N-[(1S,2R)-1-benzyl-3-{[(1S)-2-(cyclohexylamino)-1-methyl-2-oxoethyl]amino}-2-hydroxypropyl]-3-(pentylsulfonyl)benzamide 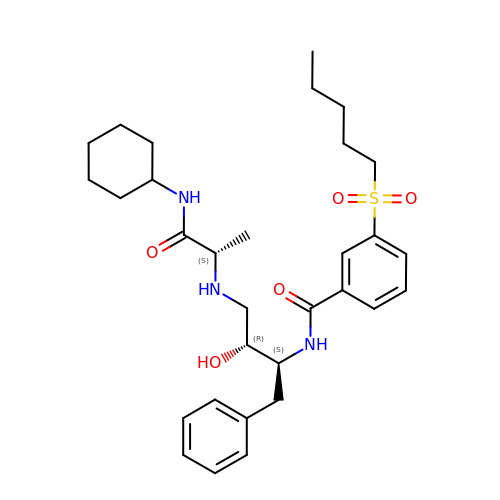| C31 H45 N3 O5 S | FBMGVFBNGKNQCB-WTWMYVDVSA-N[1-TERT-BUTYL-3-(2,4-DICHLOROPHENYL)-5-HYDROXY-1H-PYRAZOL-4-YL][2-CHLORO-4-(METHYLSULFONYL)PHENYL]METHANONE 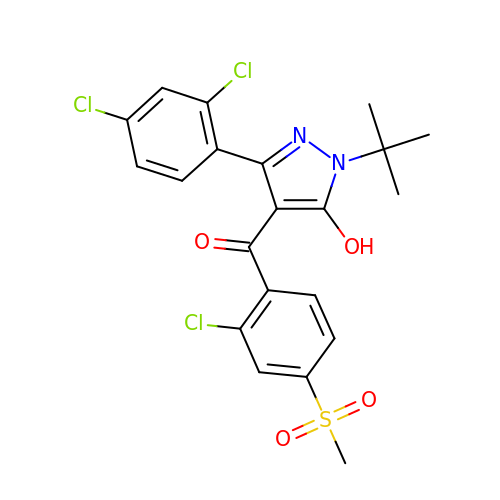| C21 H19 Cl3 N2 O4 S | HVZVWLVEDDWLOA-UHFFFAOYSA-N> SNLYTERVLSVHHWNDTLFSFKTTRNPGLRFKTGQFVMIGLEVDGRPLMRAYSIASPNYEEHLEF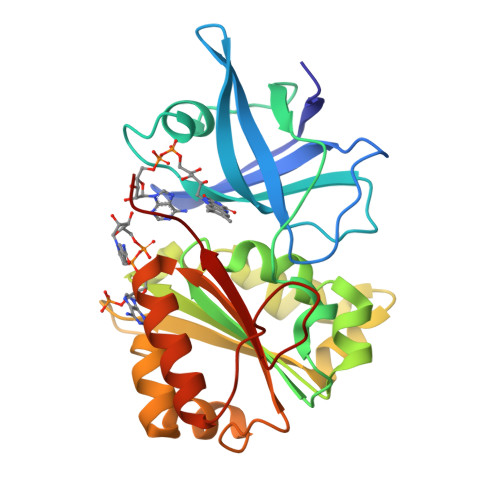FSIKVPDGPLTSRLQHLKEGDELMVSRKPTGTLVHDDLLPGKHLYLLSTGTGMAPFLSVIQDPETYERYEKVILVHGVRWVSELAYADFITKVLPEHEYFGDQVKEKLIYYPLVTREPFRNQGRQTDLMRSGKLFEDIGLPPMNPQDDRAMICGSPSMLEETSAVLDSFGLKISPRMGEPGDYLIERAFVEK> MSTIFPFIGVPEDYILPKTEELPIFREVAWDFEKDEPILEKGDFKIIEKKEALKVWIYKCIKTNRYEHEIYSLEYGTELSELIGQKYTKGLTESEASRFIKEALLIN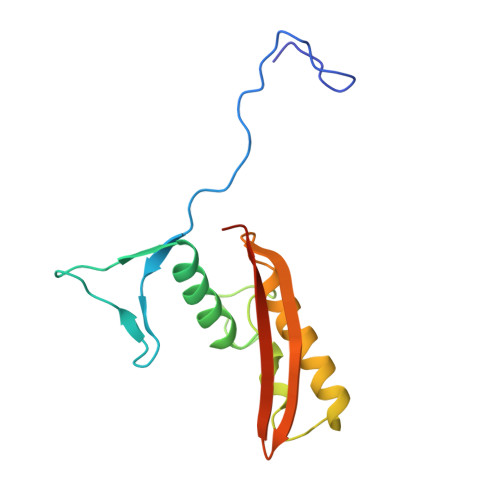PYILEVNVKSANFNRDILSANVKVSTIYGEVEINV> MYDYLFKVVLIGDSGVGKSNLLSRFTRNEFNLESKSTIGVEFATRSIQVDGKTIKAQIWDTAGQERYRRITSAYYRGAVGALLVYDIAKHLTYENVERWLKELRDHADSNIVIMLVGNKSDLRHLRAVPTDEARAFAEKNNLSFIETSALDSTNVEEAFKNILTEIYRIVSQKQIADRAAHDESPGNNVVDIS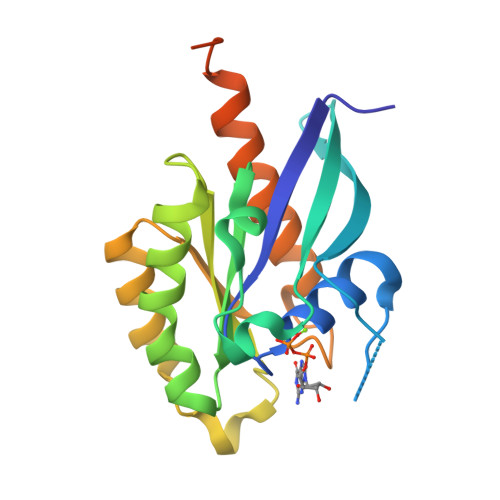VPPTTD N,N'-butane-1,4-diylbis(2,3-dihydroxybenzamide) 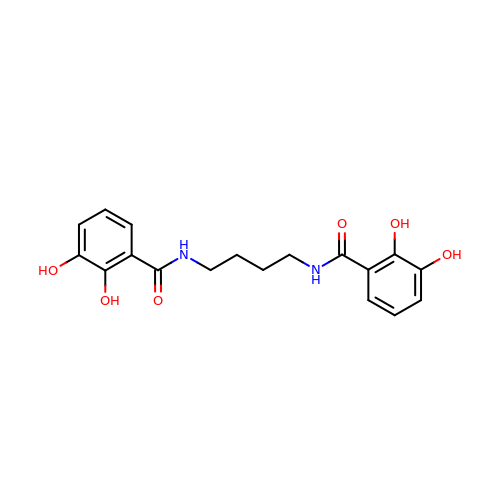| C18 H20 N2 O6 | FBRVRHJYPWFVCL-UHFFFAOYSA-N> MVQKESQATLEERESELSSNPAASAGASLEPPAAPAPGEDNPAGAGGAAVAGAAGGARRFLCGVVEGFYGRPWVMEQRKELFRRLQKWELNTYLYAPKDDYKHRMFWREMYSVEEAEQLMTLISAAREYEIEFIYAISPGLDITFSNPKEVSTLKRKLDQVSQFGCRSFALLFDDIDHNMCAADKEVFSSFAHAQVSITNEIYQYLGEPETFLFCPTEYCGTFCYPNVSQSPYLRTVGEKLLPGIEVLWTGPKVVSKEIPVESIEEVSKIIKRAPVIWDNIHANDYDQKR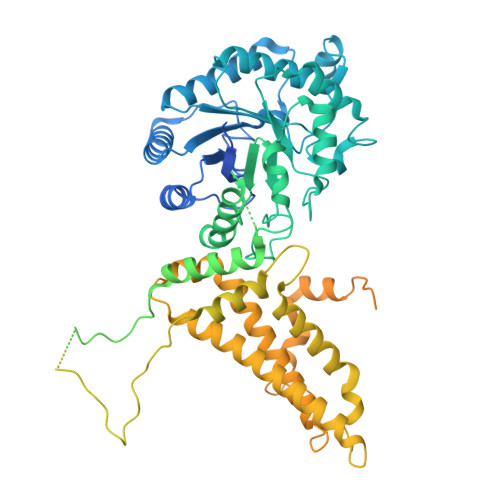LFLGPYKGRSTELIPRLKGVLTNPNCEFEANYVAIHTLATWYKSNMNGVRKDVVMTDSEDSTVSIQIKLENEGSDEDIETDVLYSPQMALKLALTEWLQEFGVPHQYSSRQVAHSGAKASVVDGTPLVAAPSLNATTVVTTVYQEPIMSQGAALSGEPTTLTKEEEKKQPDEEPMDMVVEKQEETDHKNDNQILSEIVEAKMAEELKPMDTDKESIAESKSPEMSMQEDCISDIAPMQTDEQTNKEQFVPGPNEKPLYTAEPVTLEDLQLLADLFYLPYEHGPKGAQMLREFQWLRANSSVVSVNCKGKDSEKIEEWRSRAAKFEEMCGLVMGMFTRLSNCANRTILYDMYSYVWDIKSIMSMVKSFVQWLGCRSHSSAQFLIGDQEPWAFRGGLAGEFQRLLPIDGANDLFFQPPPLTPTSKVYTIRPYFPKDEASVYKICREMYDDGVGLPFQSQPDLIGDKLVGGLLSLSLDYCFVLEDEDGICGYALGTVDVTPFIKKCKISWIPFMQEKYTKPNGDKELSEAEKIMLSFHEEQEVLPETFLANFPSLIKMDIHKKVTDPSVAKSMMACLLSSLKANGSRGAFCEVRPDDKRILEFYSKLGCFEIAKMEGFPKDVVILGRSL>[4x]GAMD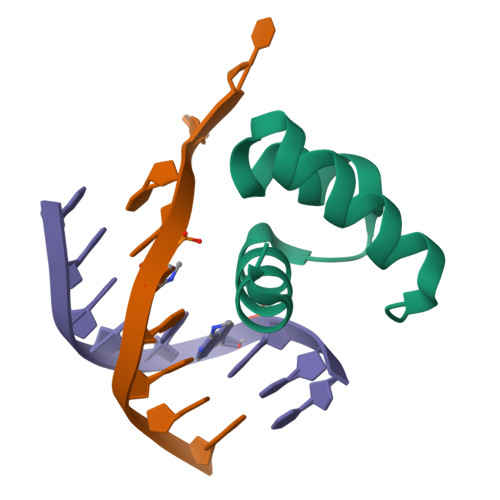MSWTDERVSTLKKLWLDGLSASQIAKQLGGVTRNAVIGKVHRLGL We describe the design, kinetic properties, and structures of engineered subtilisin proteases that degrade the active form of RAS by cleaving a conserved sequence in switch 2. The engineering process to develop specificity for the RAS sequence QEEYSAM involved extensive modification of the Bacillus protease, subtilisin BPN’16–24, a canonical serine protease in which the scissile peptide bond is attacked by a nucleophilic serine (S221). The nucleophilicity of S221 results from its interactions with the catalytic histidine (H64) and aspartic acid (D32) that together form a charge relay system. To generate high specificity for the RAS target sequence, the active site was modified to be dependent on a cofactor (imidazole or nitrite) and protease sub-sites were engineered to create a linkage between substrate and cofactor binding.

To understand the structural basis for specificity and cofactor activation, we determined crystal structures of RASProtease(I) alone, in complex with YSAM and QEEYSAM product peptides, and with imidazole. The aromatic ring of the P4 side chain has common van der Waals interactions: the Cα and Cβ atoms of A104 interact with Cε1, the Cδ1 of L126 interacts with Cδ2, and Cβ of S128 interacts with Cδ2 and Cε2. Because of the space created in the S4 pocket by the L135V mutation, either a water or an ion coordinates the hydroxyl of P4 Tyr, the hydroxyl of Y171, and the backbone nitrogen of S132 in RASProtease(I). We currently have this modeled as a chloride ion based on the peak height observed in an anomalous difference fourier map; however, added chloride does not appear to influence kinetic properties. P4 interactions are facilitated by a significant shift of the loop containing residues 130 to 133 of RASProtease(I) relative to the Protease1(N) complex. Mutation of S101K increases activity with Ser at the P3 position. Hydrogen bonding interactions between the backbone nitrogen and carbonyl oxygen of the P3 residue and the corresponding partners on residue G127 are conserved. Structures with a cognate peptide bound show that the L135V mutation allows space for an adventitious ion-binding site that coordinates the hydroxyl group of the P4 tyrosine of the substrate. This stabilizing interaction may be an important element for rescuing the active conformation of the catalytic region and enabling strong cofactor activation.

> YSAM;> AKCVSYGVAQIKAPALHSQGYTGSNVKVAILDTGIDSSHPDLNVAGGASFVPSETNPFQDNSSGGTHIAGTVLAVAPSASLYAVKVLGADGKGQASWIINGIEWAIANNMDVINMSLGSPSGSAAVKAAVDKAVASGVVVVAAAGNSGTSGSSSTVTYPAKYPSVIAVGAVDSSNQRAPFSSVGPELDVMAPGVSICSTLPGGKYGALSGTSMASPHVAGAAALILSKHPNWTNTQVRSSLENTATKLGDSFYYGKGLINVEAAAQ>MTTKNTLQPTEAAYIAGFLDGDGSIYARLIPRPDYKDIKYQVELAISFIQRKDKFPYLQDIYDQLGKRGTLRKDRGDGIADYTIWGSTHLSI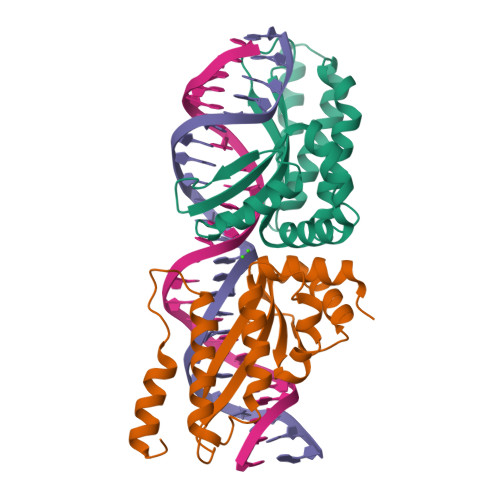ILPDLVPYLRIKKKQANRILHIINLYPQAQKNPSKFLDLVKIVDDVQNLNKRADELKSTNYDRLLEEFLKAGKIESSP[4x]> GPLGSDHGETLCGACGDSDG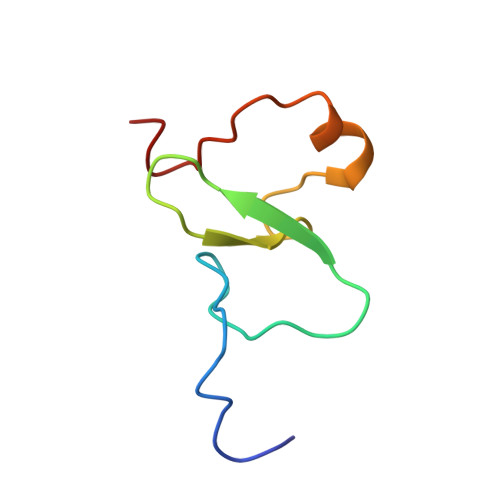ADEFWICCDLCEKWFHGKCVKITPARAEHIKQYKCPSCSN>HMLEGGSGGSGGSTIYHAKDAVQATKPDMRKPRLVVFVVGETARADHVSFNGYERDTFPQLAKIDGVTNFSNVTSCGTSTAYSVPCMFSYLGADEYDVDTAKYQENVLDTLDRLGVSILWRDNNSDSKGVMDKLPKAQFADYKSATNNAICNTNPYNECRDVGMLVGLDDFVAANNGKDMLIMLHQMGNHGPAYFKRYDEKFAKFTPVCEGNELAKCEHQSLINAYDN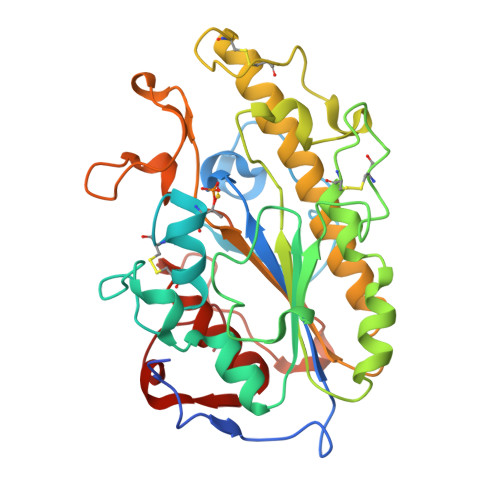ALLATDDFIAQSIQWLQTHSNAYDVSMLYVSDHGESLGENGVYLHGMPNAFAPKEQRSVPAFFWTDKQTGITPMATDTVLTHDAITPTLLKLFDVTADKVKDRTAFIR[2x]> GAAQTNTLSENTNQSAAELVKNLYNTAYKGEMPQQAQGLTINKSTKGDVHAAFGEPERPVGGDNRFDLYHWNMGQPGYGFSYHKDMTISEIRYFGTGVE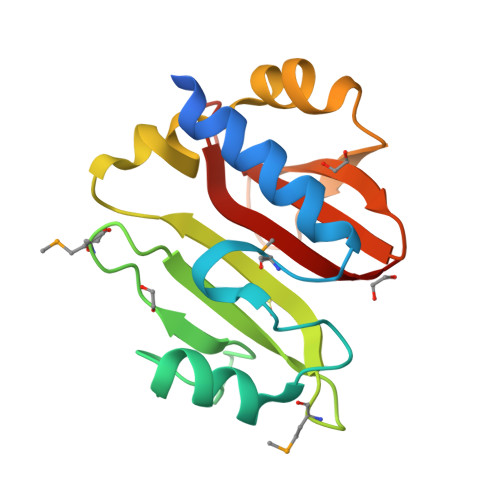RQLNLGGVTPEVLQKQLGPVNRVLTVPFTDEIDYVYDTGRYELHFVIGTDQTADHVNLKAK bis[oxidanyl-[oxidanyl-[oxidanyl(phosphonooxy)phosphoryl]oxy-phosphoryl]oxy-phosphoryl] hydrogen phosphate | H11 O28 P9 | 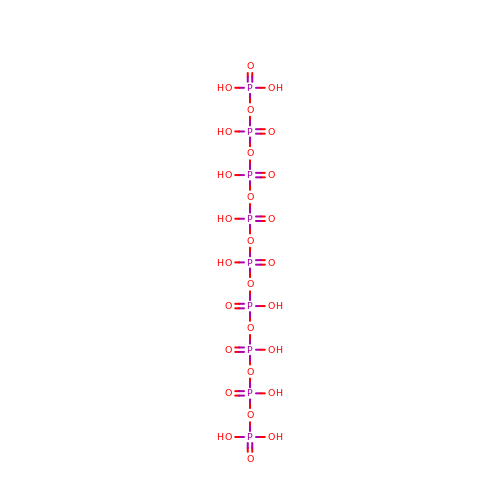CGJFWWJXTCZYEB-UHFFFAOYSA-N5-chloranyl-6-fluoranyl-3-(4-piperazin-1-yl-2-propan-2-yloxy-phenyl)-1~{H}-indole-2-carboxamide 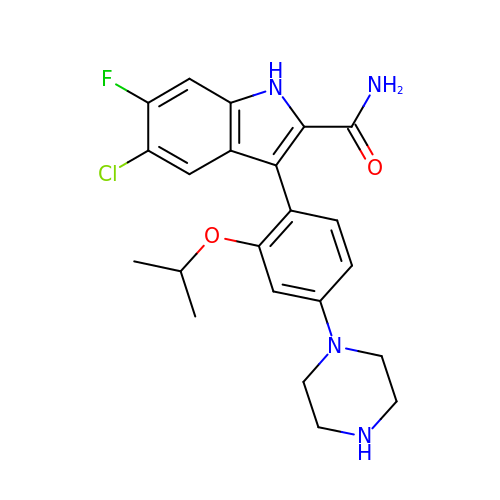| C22 H24 Cl F N4 O2 | MOVJBOWCKBGZHU-UHFFFAOYSA-N>[2x]MGSDYTSFKESKPASILVVPPLNESPDVNGTWGMLASTAAPLSEAGYYVFPAAVVEETFKQNGMTNAADIHAVRPEKLHQIFGNDAVLY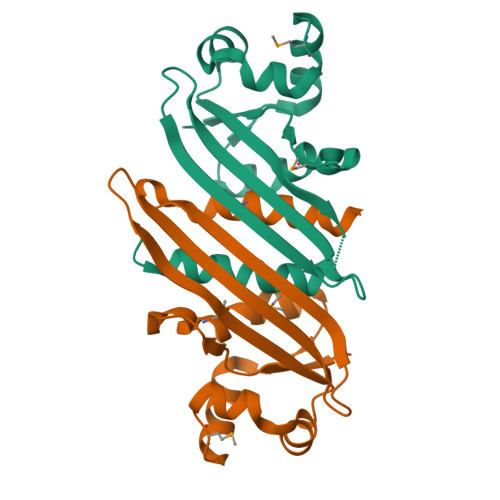ITVTEYGTSYQILDSVTTVSAKARLVDSRNGKELWSGSASIREGSNNSNSGLLGMLVSAVVNQIANSLTSLEHHHHHH>[2x]ETGKHNCFCIQEVVSGLRQPVGALHSGDGSQRLFILEKEGYVKILTPEGEIFKEPYLDIHKLVQSGIKGGDERGLLSLAFHPNYKKNGKLYVSYTTNQERWAIGPHDHILRVVEYTVSRKNPHQVDLRTARVFLEVAELHRKHLGGQLLFGPDGFLYIILGDGMITLDDMEEMDGLSDFTGSVLRLDVDTDMCNVPYSIPRS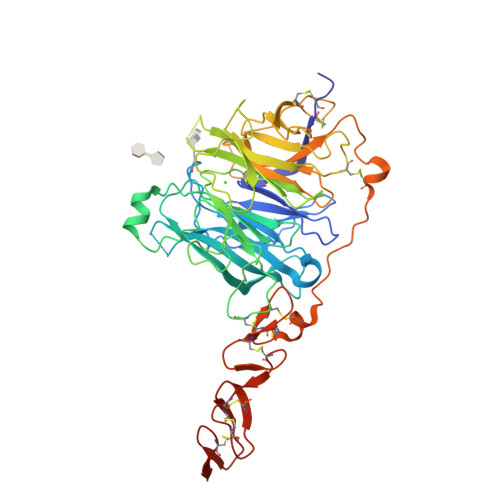NPHFNSTNQPPEVFAHGLHDPGRCAVDRHPTDININLTILCSDSNGKNRSSARILQIIKGKDYESEPSLLEFKPFSNGPLVGGFVYRGCQSERLYGSYVFGDRNGNFLTLQQSPVTKQWQEKPLCLGTSGSCRGYFSGHILGFGEDELGEVYILSSSKSMTQTHNGKLYKIVDPKRPLMPEECRATVQPAQTLTSECSRLCRNGYCTPTGKCCCSPGWEGDFCRTAKCEPACRHGGVCVRPNKCLCKKGYLGPQCEQVDGTKHHHHHH> MKLTIHEIAQVVGAKNDISIFEDTQLEKAEFDSRLIGTGDLFVPLKGARDGHDFIETAFENGAAVTLSEKEVSNHPYILVDDVLTAFQSLASYYLEKTTVDVFAVTGSNGKTTTKDMLAHLLSTRYKTYKTQGNYNNEIGLPYTVLHMPEGTEKLVLEMGQDHLGDIHLLSELARPKTAIVTLVGEAHLAFFKDRSEIAKGKMQIADGMASGSLLLAPADPIVE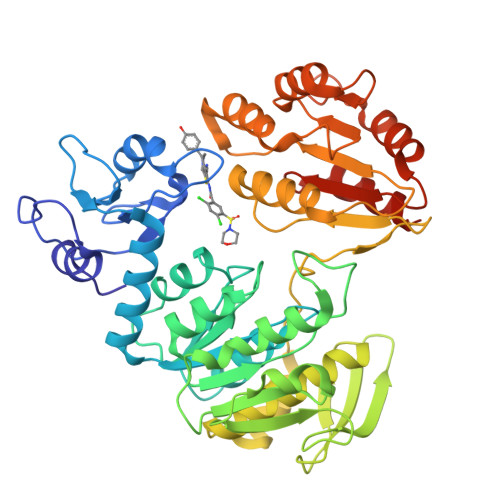DYLPIDKKVVRFGQGAELEITDLVERKDSLTFKANFLEQALDLPVTGKYNATNAMIASYVALQEGVSEEQIRLAFQHLELTRNRTEWKKAANGADILSDVYNANPTAMKLILETFSAIPANEGGKKIAVLADMKELGDQSVQLHNQMILSLSPDVLDIVIFYGEDIAQLAQLASQMFPIGHVYYFKKTEDQDQFEDLVKQVKESLGAHDQILLKGSNSMNLAKLVESLENEDKRSHHHHHH> MTNSDDDLFSEKSTSSDTQQVQNILELEAKIPDI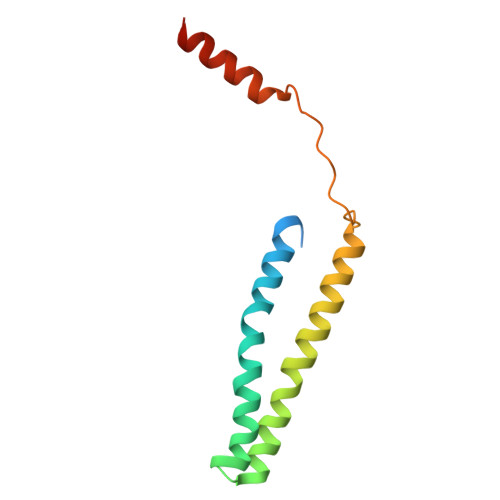LSSAGKCIEAIQLNNSLEDFRKYSKEFLETVEFISTGLRRQALELEKAEVPVVSLQPKKRYASTPLSNLIFDQSSKLIPKYC>GPLGSSDGAVTLQEYLELKKALATSEAKVQQLMKV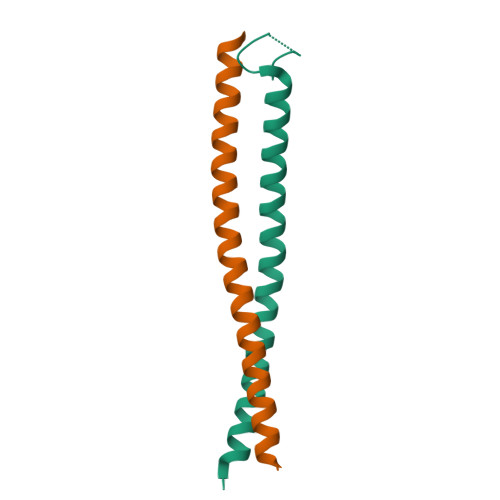NSSLSDELRKLQREIHKLQAENLQLRQP[2x]Membrane transporters belonging to the ubiquitous divalent anion/Na+ symporter (DASS) family move Krebs cycle intermediates or sulphate across the cell membrane typically by utilizing the preexisting Na+ gradient. However, like other well-characterized bacterial DASS proteins, VcINDY is known to transport succinate and other C4-dicarboxylates, rather than citrate (C6-tricarboxylate)1319. Our structure reveals a homodimeric arrangement, with each VcINDY protomer comprising eleven membrane-spanning helices (TM1–TM11), two re-entrant helix-turn-helix hairpins (HPin and HPout) and two interfacial helices (H4c and H9c). Viewed in parallel to the membrane, the VcINDY dimer is shaped like an inverted bowl with its concave mouth facing the cytoplasm, allowing the aqueous solution to reach the midpoint of the membrane.

To validate this idea as well as to gain new insights into the mechanism of human DASS, we replaced eight amino acids surrounding the citrate-binding cleft by their counterparts in NaCT, which primarily transports citrate6. We crystallized this octuple mutant of VcINDY, denoted MT5, in complex with citrate and determined the crystal structure. Although the MT5 structure remains similar to that of VcINDY, one important difference centres on the pro-S carboxylate of the bound citrate. Specifically, the side-chain hydroxyl of S200T and the backbone amide of P201G in MT5 each donate an H-bond to the pro-S carboxylate, whereas the side chain of T379V makes van der Waals interactions with the citrate. In contrast to that in VcINDY, the pro-S carboxylate latches onto the amino ends of TM5b and the second helix in HPout in MT5, with its putative negative charge stabilized by the positive helix dipoles (crystallization pH∼7). Since NaCT transports the trianionic citrate6, our structure may foretell the interactions between NaCT and its bound substrate. Specifically, 95 mM citrate reduced the succinate transport rate by <20% in VcINDY, whereas a mere 10 mM citrate decreased the transport rate by >40% in MT5 (at pH 7.4). Since VcINDY and MT5 were inserted into the liposome membrane in presumably two orientations, our data suggested that the membrane-embedded MT5 interacts with trianionic citrate more strongly than VcINDY in both the inward- and outward-facing states. This stark difference is likely attributed to the altered pose of the pro-S carboxylate seen in MT5. In support of this notion, the temperature factors for the bound citrate in MT5 are lower than those in VcINDY, arguing that the citrate was more firmly bound to MT5 than VcINDY at pH∼7. On the other hand, given the amino-acid sequence similarity between VcINDY and NaCT as well as the homologue swap mutations carried by MT5, MT5 likely recapitulates the substrate-binding properties of NaCT considerably.

>[4x]LHRNSLIVLADVALFLALYHFLPFEHNVVLGISMLAFIAVLWLTEALHVTVTAILVPVMAVFFGIFETQAALNNFANSIIFLFLGGFALAAAMHHQGLDKVIADKVLAMAQGKMSVAVFMLFGVTALLSMWISNTATAAMMLPLVLGVLSKVDADKQRSTYVFVLLGVAYSASIGGIATLVGTGPNAIAAAEVGLSFTDWMKFGLPTAMMMLPMAIAILYFLLKPTLNGMFELDRAPVNWDKGKVVTLGIFGLTVFLWIFSSPINAALGGFKSFDTLVALGAILMLSFARVVHWKEIQKTADWGILLLFGGGLCLSNVLKQTGTSVFLANALSDMVSHMGIFVVILVVATFVVFLTEFTSNVATTTLLIPVFATVAEAFGMSPVLLSVLIAVAASCAFMLPVATPPNAIVFASGHIKQSEMMRVGLYLNIACIGLLTAIAMLFWQ>[2x]ARKCSLTGKWTNNLGSIMTIRAVNSRGEFTGTYLTAVADNPGNITLSPLLGIQHKRASQPTFGFTVHWNFSESTTVFTGQCFIDRNGKEVLKTMWLLRS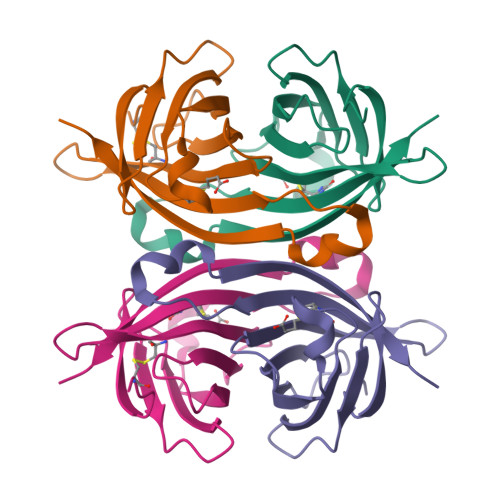SVNDISYDWKATRVGYNNFTRLSTVEE~{N}-[2-[2-fluoranyl-4-[(4-propan-2-ylpiperazin-1-yl)methyl]phenyl]pyridin-4-yl]-2-methoxy-5-morpholin-4-yl-pyridine-3-sulfonamide | C29 H37 F 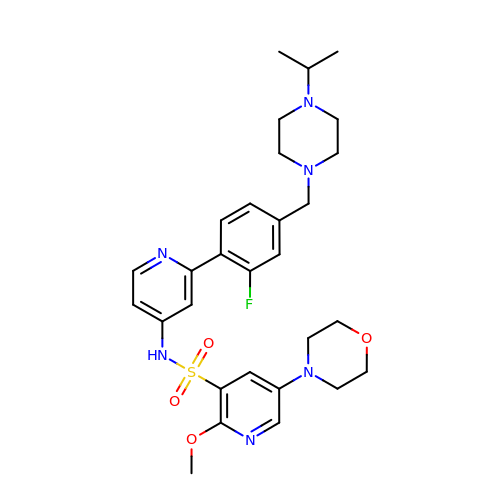N6 O4 S | ODQVPYNCHSLNGV-UHFFFAOYSA-N> MNPLYRAAIHQLFLALDLPTPNDEESVLSLQVGPHLCHLAEHPTDHLLMFTRLEGQGDATANEQ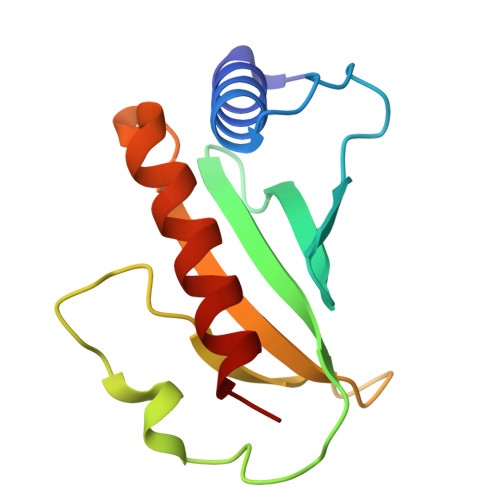NLFSQDPCKPILGRDPESGERLLWNRQPLQLLDRAQIHHQLEQLVAAAEELR>[2x]AAPDEITTAWPVNVGPLNPHLYTPNQMFAQSMVYEPLVKYQADGSVIPWLAKSWTHSEDGKTWTFTLRDDVKFSNGEPFDAEAAAENFRAVLDNRQRHAWLELANQIVDVKALSKTELQITLKSAYYPFLQELALPRPFRFIAPSQFKNH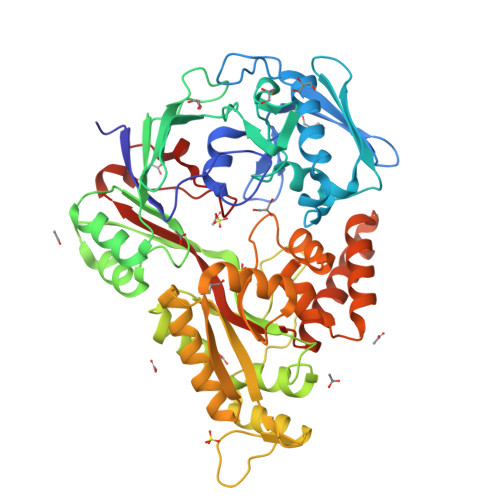ETMNGIKAPIGTGPWILQESKLNQYDVFVRNENYWGEKPAIKKITFNVIPDPTTRAVAFETGDIDLLYGNEGLLPLDTFARFSQNPAYHTQLSQPIETVMLALNTAKAPTNELAVREALNYAVNKKSLIDNALYGTQQVADTLFAPSVPYANLGLKPSQYDPQKAKALLEKAGWTLPAGKDIREKNGQPLRIELSFIGTDALSKSMAEIIQADMRQIGADVSLIGEEESSIYARQRDGRFGMIFHRTWGAPYDPHAFLSSMRVPSIADFQAQQGLADKPLIDKEIGEVLATHDETQRQALYRDILTRLHDEAVYLPISYISMMVVSKPELGNIPYAPIATEIPFEQIKPVKP4-(1,3-benzothiazol-2-yl)-4-hydroxycyclohexa-2,5-dien-1-one | C13 H9 N O2 S | 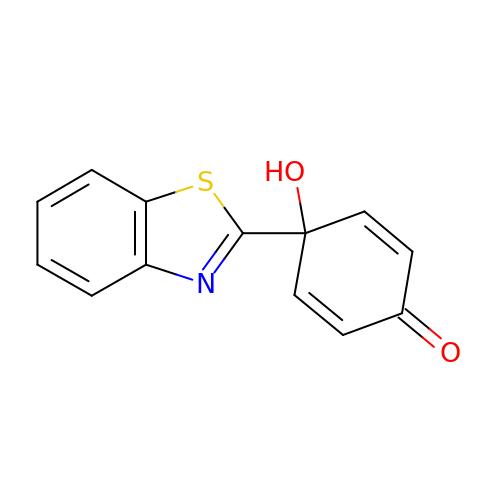SDYBYKXWYDVVKP-UHFFFAOYSA-N We describe here the high‐resolution crystal structures of GM from Clostridium cochlearium, reconstituted with AdoMeCbl and AdoEtCbl and the pseudo‐substrate (S,S)‐tartrate. As previously observed, GM forms a hetero‐tetramer consisting of two copies of the larger ϵ‐subunit (an (αβ)8 TIM‐barrel) and the smaller B12‐binding σ‐subunit, showing a typical Rossman fold. The ϵ‐subunit harbours the substrate‐binding site comprising three arginine residues (the “arginine claw”) that undergo strong polar binding interactions with the carboxylate groups of an (S,S)‐tartrate ion. The process catalysed by GM [12a] assigns the enzyme‐generated Ado‐radical the specific function of abstracting (in the direction from (S)‐glutamate to (2S,3S)‐3‐methylaspartate) the pro‐S H‐atom from the 4‐position of (S)‐glutamate, furnishing 5′‐deoxyadenosine and a 4‐glutamyl radical.

We have set out to test this AdoCbl‐activation hypothesis with two “stretched” AdoCbl‐homologues, designed and synthesised as potential structural mimics of “activated” AdoCbl, provisionally named “homocoenzyme B12” (AdoMeCbl) and “bis‐homocoenzyme B12” (AdoEtCbl). AdoMeCbl and AdoEtCbl are bound in a base‐off/His‐on form, with distances between cobalt and the coordinating histidine imidazole of 2.21 Å and 2.17 Å, respectively, similar to GM‐bound AdoCbl (2.22 Å) and free AdoMeCbl (2.19 Å). In both new structures, the electron density for the “stretched” AdoCbl‐homologues indicated an intact bond between the cobalt ion and the terminal carbons C6′ or C7′ of the 5′‐methyl‐ or 5′‐ethyl‐adenosyl ligands of AdoMeCbl and AdoEtCbl, respectively. The refined Co−C bond lengths at 2.07 Å or 1.98 Å for the bound AdoMeCbl and AdoEtCbl, respectively, were somewhat longer or slightly shorter than the 2.00 Å observed in the crystal structures of AdoCbl and AdoMeCbl, [25a] but in stark contrast to distances of >3.2 Å observed between cobalt and C5′ of the adenosyl ligand in GM reconstituted with AdoCbl. The distances from Co to C5′ of the Ado moieties of the bound AdoMeCbl and AdoEtCbl were 3.2 Å and 4.2 Å, strikingly comparable to the distances between the Co‐atom and C5′ in the two observed structures of “activated” AdoCbl in the crystal structure of GM reconstituted with AdoCbl. The adenosyl moiety of the bound Cbls and its protein environment are positioned at a nearly indistinguishable location in substrate‐bound GM reconstituted with AdoCbl (GM‐AdoCbl), AdoMeCbl (GM‐AdoMeCbl), or AdoEtCbl (GM‐AdoEtCbl), clearly defining a firm H‐bonding “adenosine‐binding cavity” (ABC) that intimately interacts with the substrate‐binding site. In contrast, in GM‐AdoEtCbl, the organometallic AdoEt unit displays a ribose E1 (C1′‐exo) conformation. In the case of AdoEtCbl, an intact Co−C bond is also observed, but the E1 (C1′‐exo) ribose conformation and a strained conformation of the linker between the adenine and the ethyl‐Cbl moieties are indicated.

>[2x]MEKKTIVLGVIGSDCHAVGNKILDHAFTNAGFNVVNIGVLSPQENFIKAAIETKADAILVSSLYGQGEIDCKGLRQKCDEAGLEGILLYVGGNIVVGKQHWPDVEKRFKDMGYDRVYAPGTPPEVGIADLKKDLNIE;>MELKNKKWTDEEFHKQREEVLQQWPTGKEVDLQEAVDYLKKIPAEKNFAEKLVLAKKKGITMAQPRAGVALLDEHIELLRYLQDEGGADFLPSTIDAYTRQNRYDECENGIKESEKAGRSLLNGFPGVNHGVKGCRKVLEAVNLPLQARHGTPDSRLLAEIIHAGGWTSNEGGGISYNVPYAKNVTIEKSLLDWQYCDRLVGFYEEQGVHINREPFGPLTGTLVPPSMSNAVGITEALLAAEQGVKNITVGYGECGNMIQDIAALRCLEEQTNEYLKAYGYNDVFVTTVFHQWMGGFPQDESKAFGVIVTATTIAALAGATKVIVKTPHEAIGIPTKEANAAGIKATKMALNMLEGQRMPMSKELETEMAVIKAETKCILDKMFELGKGDLAIGTVKAFETGVMDIPFGPSKYNAGKMMPVRDNLGCVRYLEFGNVPFTEEIKNYNRERLQERAKFEGRDVSFQMVIDDIFAVGKGRLIGRPE[2x]>[2x]DYVEQR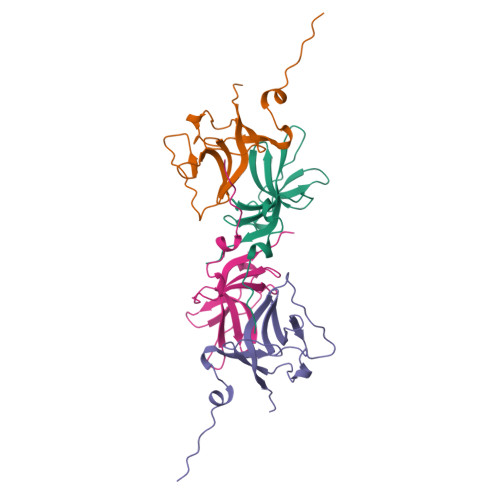IDLNQLLIQHPSATYFVKASGDSMIDGGISDGDLLIVDSAITASHGDIVIAAVDGEFTVKKLQLRPTVQLIPMNSAYSPITISSEDTLDVFGVVIHVVKAMR> GSHGNYAGNFSGSSRDICLDGARLRAECRRGDGGYSTSVIDLNRYLSNDNGHFRWVSTATVTVQQGDTLRDIGRRFDCDFHEIARRNNIQNEDLIYPGQVLQVGGNFWDSARDVRLVDGGKVLEAELR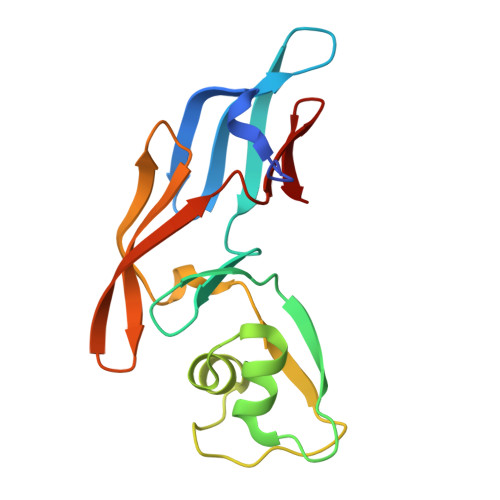YSGGWNRSRIYLDEHIGNRNGELIHC>[2x]MGSHHHHHHDITSLYKKAGSAAAVLEENLYFQGSFTMLHEIPKSEILKELKRIGAKRVLIQSPEGLRREAEELAGFLEENNIEVFLHGEINYGACDPADREAKLVGCDALIHLGHSYMKLPLEVPTIFVPAFARVSVVEALKENIGEIKKLG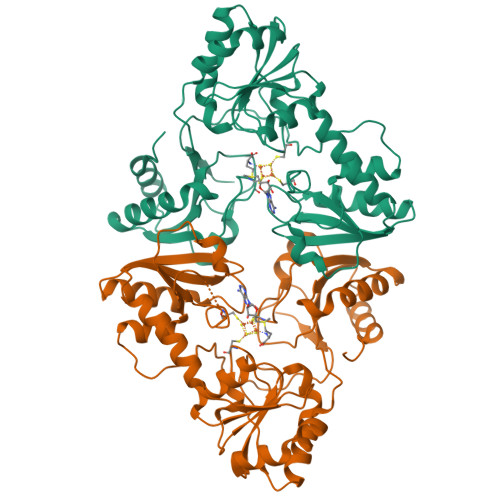RKIIVTTTAQHIHQLKEAKEFLESEGFEVSIGRGDSRISWPGQVLGCNYSVAKVRGEGILFIGSGIFHPLGLAVATRKKVLAIDPYTKAFSWIDPERFIRKRWAQIAKAMDAKKFGVIVSIKKGQLRLAEAKRIVKLLKKHGREARLIVMNDVNYHKLEGFPFEAYVVVACPRVPLDDYGAWRKPVLTPKEVEILLGLREEYEFDEILGGPRESDEPFGISIHSTR>[4x]LEINHQEEPGFEVITRIDLGIRPEIQRGEPVSIERWSQCMDAEGKVLDPENVKKLIFRGGLCHAVRKLTW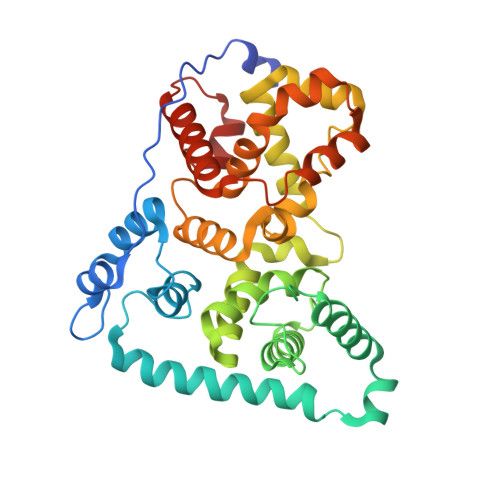KFLLNYFPWDSSKEDRRLLIKRKTDEYFRMKLQWKSVSEEQEKRNTRLKDYKSLIEKDVNRTDRTNPFYEGHENPGLILLHDILMTYCMYDFDLGYIQGMSDLLSPILYVMENEVDAFWCFVAFIEQMHCNFEEQMQGMKTELSQLSTLLKLLDLGFWNYLESQESGYLYFCFRWLLIRFKREFNFQDTLRLWEVMWTGLPCQNFHLLICCAILDSEKQKIMENHYGFNEILKHINELSLKLDVEEVLCKAEAIYCQMMKCKDLPQAVGEILGLKDST O-(((1R)-((N-PHENYLMETHOXYCARBONYL-L-ALANYL)AMINO)ETHYL)HYDROXYPHOSPHONO)-L-BENZYLACETIC ACID | C22 H27 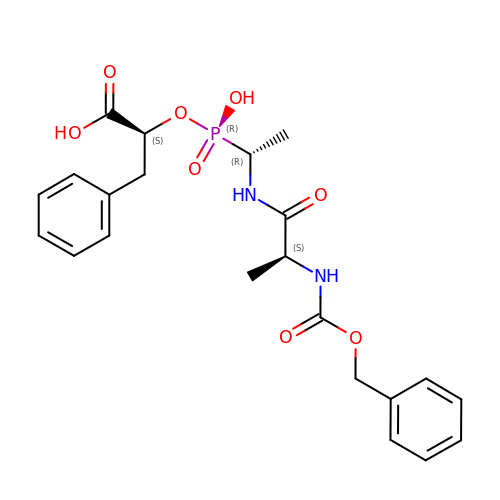N2 O8 P | UPJNMOBJDSFRTI-FCEWJHQRSA-N>PAMTNIVLRDDQTSVATKTLIPIVSDGNMSVWRENAANVPIDGQIKLTGQWERMKDGTYRLNAKLEVPVMETAGAGGAYVAPPKVAYKVTASLTLYAPSRSTIADRANAMKMLSAVLCGADATAGTTLSPQSVTGDAWKNSALPFVFG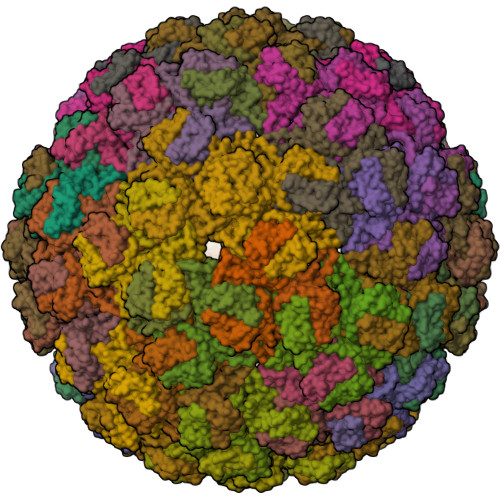FINQAFPT[90x]>QDINAQLTTWFSQRLAGFSDEVVVTLRSSPNLLPSCEQPAFSMTGSAKLWGNVNVVARCANEKRYLQVNVQATGNYVAVAAPIARGGKLTPANVTLKRGRLDQLPPRTVLDIRQIQDAVSLRDLAPGQPVQLTMIRQAWRVKAGQRVQVIANGEGFSVNAEGQAMNNAAVAQNARVRMTSGQI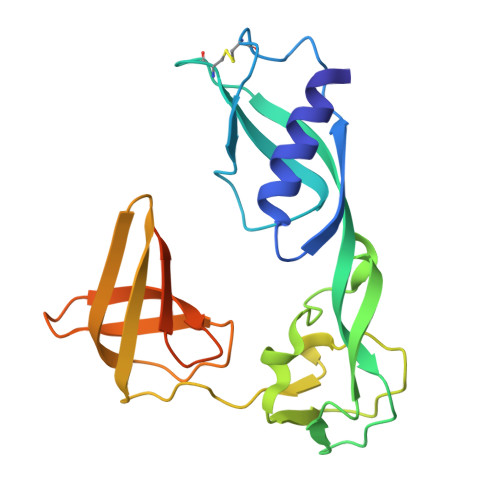VSGTVDSDGNILINLDPNSSSVDKLAAALEHHHHHH[4x]>GSHMTYPKYLLSPETIEALRKPTFDVWLWEPNEMLSCLEHMYHDLGLVRDFSINPVTLRRWLFCVHDNYRNNPFHNFRHCFCVAQMMYSMVWLCSLQEKFSQTDILILMTAAICHDLDHPGYNNTYQINARTELAVRYNDISPLENHHCAVAFQILAEPECNIFSNIPPDGFKQIRQGMITLILATDMARHAEIMDSFKEKMENFDYSNEEHMTLLKMILIKCCDISNEVRPMEVAEPWVDCLLEEYFMQSDREKSEGLPVAPFMDRDKVTKATAQ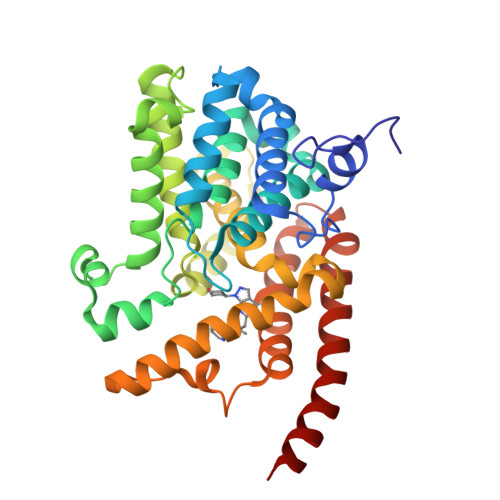IGFIKFVLIPMFETVTKLFPMVEEIMLQPLWESRDRYEELKRIDDAMKELQKK[2x]Here we describe extendable linear, curved and angled protein building blocks, as well as inter-block interactions, that conform to specified geometric standards; assemblies designed using these blocks inherit their extendability and regular interaction surfaces, enabling them to be expanded or contracted by varying the number of modules, and reinforced with secondary struts. We construct twistless helix repeat (THR) protein blocks from identical straight α-helices (typically 2–4 helices in each unit); the length of the blocks can be varied simply by varying the number of repeat units. Restricting helical geometry to ideal straight helices with zero helical twist in principle considerably limits what types of structure could be built, but this is more than compensated by the great simplification of downstream material design, as illustrated below. Using X-ray crystallography and electron microscopy, we validate nanomaterial designs ranging from simple polygonal and circular oligomers that can be concentrically nested, up to large polyhedral nanocages and unbounded straight ‘train track’ assemblies with reconfigurable sizes and geometries that can be readily blueprinted.

To generate straight, linear THRs, we set Δθ to zero. This results in perfectly straight repeat proteins in which each repeat unit is translated but not rotated relative to the previous unit. We tested 33 linear THRs (with Δh = 0) with helices either about 20 or about 40 residues in height; 23 of 33 tested designs were solubly expressed, and 13 of 19 designs analysed by SEC were primarily monomeric as designed. As for all of the THR blocks described here, because of the ideality of the block construction, the same sequence interactions can be used for the intra-block and inter-block interactions; we refer to blocks in which the terminal repeats have identical sequences to the internal repeats as uncapped, and those in which the terminal helices have polar outward-facing residues to prevent self-association (like the linear blocks above) as capped. a,b, The linear THR designs (rainbow) are nearly identical to the experimentally determined structures (grey). Side-chain sticks between α-carbon and β-carbon are shown to indicate helical phasing. a, Left: the 2.5-Å-resolution crystal structure of the short, linear THR1 has a 0.8 Å CA RMSD to the design.

> HHHHHHSGSGENLYFQGSGSEEIVEEAETALKALLEEAEKGGKEDALEIAEKLAELAKEALEVLLEAGASPELIVRLAETALKALLAIAELGGEELALEIARILAELAEVALEVLLELGASPELIVRLAETALEALLAIARLGGEELALEIARILAELAEVALEVLLELGASPELIKKLAETAEEALEAIAKLGGEELAEEIAKILAELAEVAKEVQKELGAS>AHHHHHHGSIDLILLAGKLKRIPRMGWLIKGVPNPESVADHSYRVAFITLLLAEELKKKGVEIDVEKALKIAIIHDLGEAIITDLPLSAQKYLNKEEAEAKALKDVLPEYTELFEEYSKALTLEGQLVKIADKLDMIIQAYEYELSGAKNLSE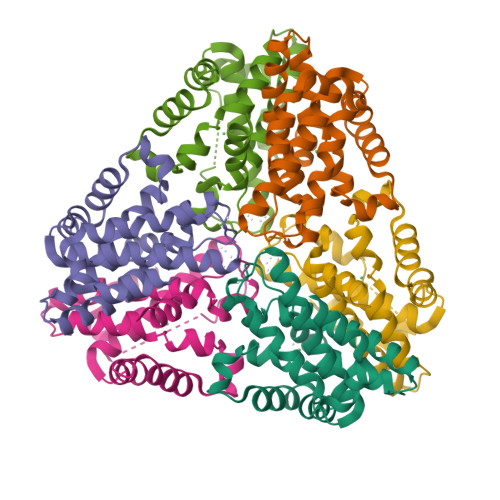FWNALEDLEKLEISRYLREIIEEVRRLKDDH[6x]(4aR,7aR)-7a-[(1R,2R)-2-(2-{[(1R,2R)-2-methylcyclopropyl]methoxy}propan-2-yl)cyclopropyl]-6-(pyrimidin-2-yl)-4,4a,5,6,7,7a-hexahydropyrrolo[3,4-d][1,3]thiazin-2-amine | C21 H31 N5 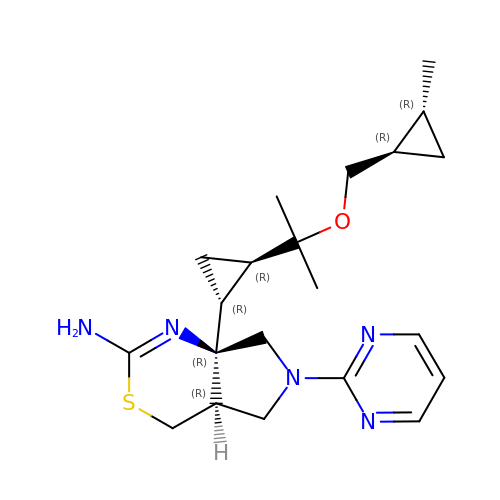O S | BFGQEVKVRRYAQC-IFEDNLKFSA-N>MPFTYSIEATRNLATTERCIQDIRNAPVRNRSTQFQLAQQNMLAYTFGEVIPGFASAGINGMDYRDVIGRPVENAVTEGTHFFRDDFRVDSNAKAKVAGDIFEIVSSAVMWNCAARWNSLMVGEGWRSQPRYSRPTLSPSPRRQVAVLNLPRSFDWVSLLVPESQEVIEEFRAGLRKDGLGLPTSTPDLAVVVLPEEFQNDEMWREEIAGLTRPNQILLSGAYQRLQGRVQPGEISLAVAFKRSLRSDRLYQPLYEANVMQLLLEGKLGAPKVEFEVHTLAPEGTNAFVTYEAASLYGLAEGRSAVHRAIRELYVPPTAADLARRFFAFLNERMELVNGENLYFQSHHHHHH[2x]

For the filament-forming sequence-specific DNA endonuclease SgrAI, the process of filamentation both accelerates its DNA cleavage activity and expands its DNA sequence specificity, thus allowing for many additional DNA sequences to be rapidly cleaved. Under basal conditions, SgrAI is a homodimeric and sequence-specific restriction endonuclease of 74 kDa with two active sites, one in each subunit. Each active site cleaves bound duplex DNA containing any one of 17 different 8 bp recognition sites. Three of these sites, known as primary sequences or primary sites, have the pattern CRCCGGYG (where R = A or G and Y = C or T) and can be cleaved by SgrAI in the absence of filamentation.

First, we present the cryo-EM structure of filamentous SgrAI bound to intact primary site DNA and Ca2+ resolved to ∼2.5 Å within the catalytic center, which represents the trapped enzyme–DNA complex prior to the DNA cleavage reaction. For the rest of the work, we refer to the model derived from this sample as SgrAISP/FCA to indicate that this particular structure is filamentous and contains an intact SP, owing to the fact that the cleavage reaction was stalled through the use of Ca2+. A total of three Ca2+ ions are located in each active site of the SgrAI dimer in sites A, B, and D. The absence of the SP in the prior structure (i.e., SgrAIno−SP/FMG) captured Mg2+ binding at one of the two metal ion sites (site A), but no metal ion binding was seen in site B. In the current structure, utilizing Ca2+, we observe occupation of both expected metal ion–binding sites. Consistent with our hypothesis, the current structure containing the SP indeed now shows a metal ion bound in site B. This Ca2+ ion forms interactions with the SP as expected, as well as with the carbonyl oxygen of Thr186, as predicted; however, the latter interaction is mediated through a water molecule rather than through direct ligation. In addition, a water molecule ligated to the site A Ca2+ is in the expected position of the nucleophile of the hydrolysis reaction catalyzed by SgrAI (dark blue sphere). The largest difference in stacking surface area of the DNA bases in the two structures is found at the second base step, between Ade2 and Cyt3 (i.e., CACCGGTG), which shows a >250% increase in stacking surface area of the ring atoms in the filamentous form (SgrAISP/FCA). Specifically, the conformation observed in SgrAISP/FCA, containing the SP, brings the carbonyl oxygen of Gly284 within 4.1 Å of the C5 atom of Cyt1 of the DNA (blue).> GADDDKPIQVNQLPQTAQTFIKTHFPDNKVAMAKMETDWFDKSYDVIFT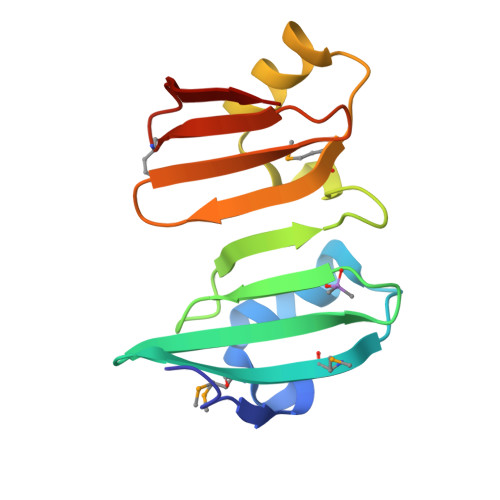NGDKLEFDKKGIWTEVNCKYSAVPVAVVPDAIKKYVATNYPDAKMLKIERDKHDYEVKLSNGWEIKFDMQFNVIDIDN> MTELETAMGMIIDVFSRYSGSEGSTQTLTKGELKVLMEKELP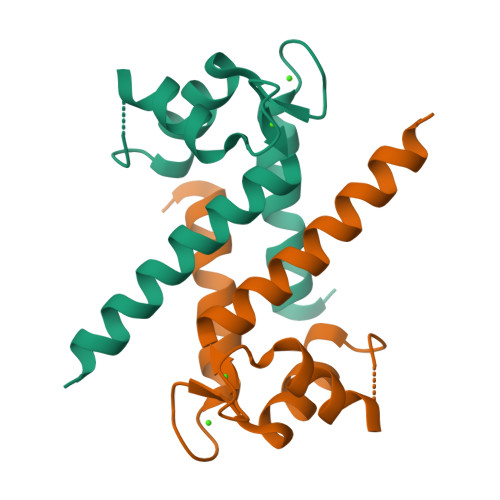GFLQSGKDKDAVDKLLKDLDANGDAQVDFSEFIVFVAAITSACHKYFEKAGLK>[4x]LAAAMLNLENKTYVIMGIANKRSIAFGVAKVLDQLGAKLVFTYRKERSRKELEKLLEQLNQPEAHLYQIDVQSDEEVINGFEQIGKDVGNIDGVYHSIAFANMEDLRGRFSETSREGFLLAQDISSYSLTIVAHEAKKLMPEGGSIVATTYLGGEFAVQNYNVMGVAKASLEANVKYLALDLGPDNIRV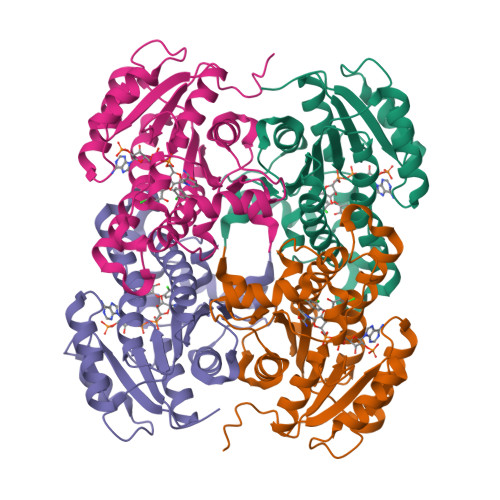NAISAGPIRTLSAKGVGGFNTILKEIEERAPLKRNVDQVEVGKTAAYLLSDLSSGVTGENIHVDSGFHAIK> MFISRHSGEGKFLFIDQRATLVIGFLPQEILGTSFYEYFHNEDIAALMESHKMVMQVPEKVTTQVYRFRCKDNSYIQLQS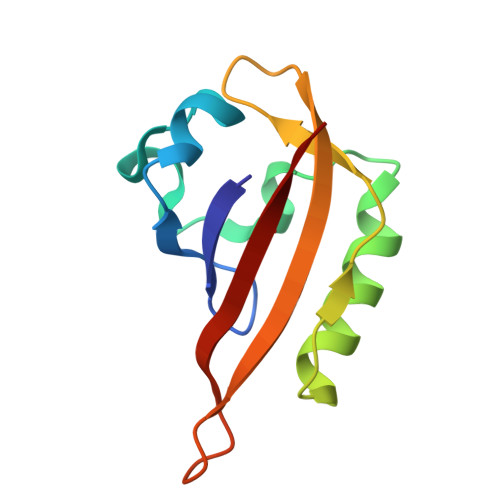EWRAFKNPATSEIDYIIAKNSVF>[5x]MVRTTKTSMAAASTVAPEVAMDEGSPSTSQAQVELPRNLEVFNEACGHVFGSSFNREDNSVISDAAAFLFKMHTHSLDGQEAKVLRASEKKRERENAKKSRKAPEAGMRVGRSLILTSRWTEYCATCVPALGSKMKVIKASGDAAMIQMMKDHNSLLRVCVRIEVWKARYVSLVALDERIQTLE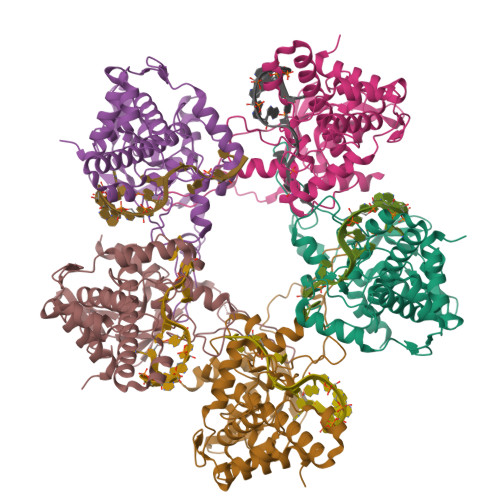DAQWFPYLSGDSYRACPGLVGGYFAKKAAAGERGKNYKKLNQTAIIPPPRFLIIGHRLQIGDQVTLRELLASIAWGLCDGVLAECWSPSQGDGSIGVVVGLPLQATGSCFLVVASHGLSAIADSRIEGTGNTNLLEECIAIQKQDGVIKCKRSGKSLYHCLKETAGAVGR>[2x]ANPLYQKHIISINDLSRDDLNLVLATAAKLKANPQPELLKHKVIASCFFEASTRTRLSFETSMHRLGASVVGFSDSANTSLGKKGETLADTISVISTYVDAIVMRHPQEGAARLATEFSGNVPVLNAGDGSNQHPTQTLLDLFTIQETQGRLDNLHVAMVGDLKYGRTVHSL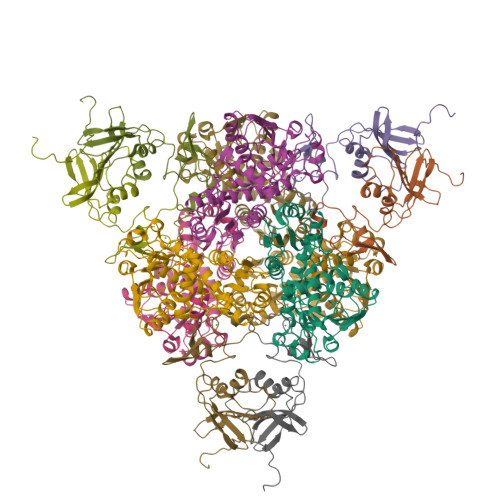TQALAKFDGNRFYFIAPDALAMPQYILDMLDEKGIAWSLHSSIEEVMAEVDILYMTRVQKERLDPSEYANVKAQFVLRASDLHNAKANMKVLHPLARVDEIATDVDKTPHAWYFQQAGNGIFARQALLALVLNRDLVL;>[2x]MTHDNKLQVEAIKRGTVIDHIPAQIGFKLLSLFKLTETDQRITIGLNLPSGEMGRKDLIKIENTFLSEDQVDQLALYAPQATVNRIDNYEVVGKSRPSLPERIDNVLVCPNSNCISHAEPVSSSFAVRKRANDIALKCKYCEKEFSHNVVLAN> MKKVMLATALFLGLTPAGANAADLGHQTLGSNDGWGAYSTGTTGGSKASSSNVYTVSNRNQLVSALGKETNTTPKIIYIKGTIDMNVDDNLKPLGLNDYKDPEYDLDKYLKAYDPSTWGKKEPSGTQEEARARSQKNQKARVMVDIPANTTIVGSGTNAKVVGGNFQIKSDNVIIRNIEFQDAYDYFPQWDPTDGSSGNWNSQYDNITINGGTHIWIDHCTFNDGSRPDSTSPKYYGRKYQHHDGQTDASNGANYITMSYNYYHDHDKSSIFGSSDSKTSDDGKLKITLHHNRYKNIVQKAPRVRFGQVHVYNNYYEGSTSSSSYPFSYAWGIGKSSK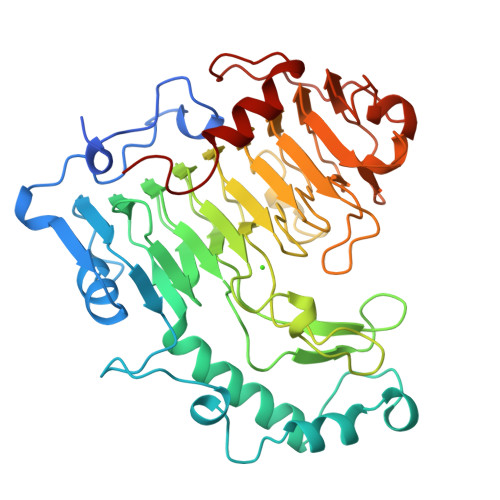IYAQNNVIDVPGLSAAKTISVFSGGTALYDSGTLLNGTQINASAANGLSSSVGWTPSLHGSIDASANVKSNVINQAGAGKLN Avapritinib is the only potent and selective inhibitor approved for the treatment of D842V-mutant gastrointestinal stromal tumors (GIST), the most common primary mutation of the platelet-derived growth factor receptor α (PDGFRA). Against this background, we solve the crystal structures of avapritinib in complex with wild-type and mutant PDGFRA and stem cell factor receptor (KIT), which provide evidence and understanding of inhibitor binding and lead to the identification of a sub-pocket (Gα-pocket). Furthermore, we report the identification of a sub-pocket (Gα-pocket) located in the N-lobe of the kinase domain, which is surrounded by amino acids of key regulatory elements such as the Gly-rich loop and the αC-helix.

Intense screening and optimization resulted in two complex structures with avapritinib in wt and gatekeeper-mutant KIT-T670I. As anticipated, a water-mediated interaction of Thr670 of KIT-wt and the N4 of the pyrrolotriazine scaffold is clearly visible in this structure. In contrast to the published working hypothesis, the water molecule thus forms a polar contact with Thr670 instead of a water network involving the catalytic lysine and the gatekeeper mutation, which results in a loss of an important interaction. Finally, comparing the binding modes of avapritinib in PDGFRA and KIT, it is striking that the interaction of the catalytic lysine (Lys627 in PDGFRA, Lys623 in KIT) with the pyrimidine was not observed in KIT. Additional water-mediated interactions were identified in KIT linking the ligand’s primary amine and Lys623 and Asp810. Apart from this, the mode of binding is very similar, and almost all interactions described for PDGFRA are also evident in KIT. Interestingly, we observed that the Gα-pocket addressed by avapritinib appears to manifest only upon ligand binding. Thus, our detailed analysis showed that the binding of avapritinib to a DFG-in, but αC-helix-out conformation characterizes it as a type 1.5 inhibitor rather than a canonical type 1 inhibitor.

>GSMPMYEVQWKVVEESNGNNYSYIDPTQLPYDHKWEFPRNRLSFGKTLGAGAFGKVVEATAQGLIKSDAAMTVAVKMLKPSAHSTEREALMSELKVLSYLGNHENIVNLLGACTHGGPTLVITEYCCYGDLLNFLRRKRDEFVPYKVAPEDLYKDFLTLEHLLSFSYQVAKGMAFLASKNCIHRDLAARNILLTHGNITKICDFGLARDIKNDSNYVDKGNARLPVKWMAPESIFNSVYTFESDVWSYGIFLWELFSLGSSPYPGMPVDSKFYKMIKEGFRMSSPEYAPAEMYDIMKTCWDADPDKRPTFKQIVQDIEKQISESTNH[2x]> GPVCEIDVILNDAESRKTAELKTEEGKLEKHYLFYDGESVSGKVNINVKQTSKRLEHQGIRIEFVGQIELFSDKSNTHEFVNLVKELALPGELTQNRSYDFEFMQVEKPYESYVGANVRLRYFLKV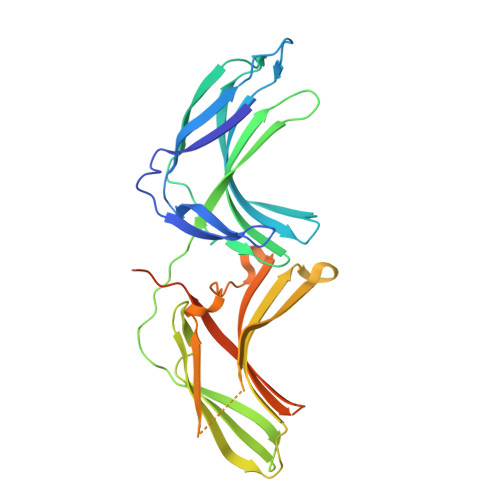TIVRRLSDLVKEYDLIVHQLATYPDVNNSIKMEVGIEDCLHIEFEYNKSKYHLKDVIVGKIYFLLVRIKIQHMELQLIKKEMTGIGPSTTTETETVAKYEIMDGAPVKGESIPIRLFLAGYDLTPTMRDVNKKFSVRYFLNLVLVDEEDRRYFKQQEIVLWRKAPEKMRKRNFHQRYESPEPRPSLSAEQPEM> MPPGVDCPMEFWTKEENQSVVVDFLLPTGVYLNFPVSRNANLSTIKQLLWHRAQYEPLFHMLSGPEAYVFTCINQTAEQQELEDEQRRLCDVQPFLPVLRLVAREGDRVKKLINSQISLLIGKGLHEFDSLCDPEVNDFRAKMCQFCEEAAARRQQLGWEAWLQYSFPLQLEPSAQTWGPGTLRLPNRALLVNVKFEGSEESF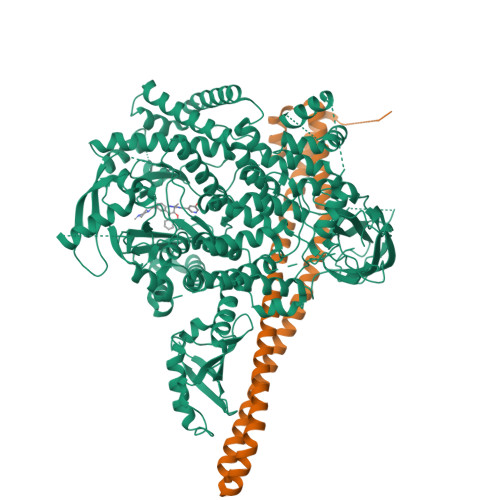TFQVSTKDVPLALMACALRKKATVFRQPLVEQPEDYTLQVNGRHEYLYGSYPLCQFQYICSCLHSGLTPHLTMVHSSSILAMRDEQSNPAPQVQKPRAKPPPIPAKKPSSVSLWSLEQPFRIELIQGSKVNADERMKLVVQAGLFHGNEMLCKTVSSSEVSVCSEPVWKQRLEFDINICDLPRMARLCFALYAVIEKAKKARSTKKKSKKADCPIAWANLMLFDYKDQLKTGERCLYMWPSVPDEKGELLNPTGTVRSNPNTDSAAALLICLPEVAPHPVYYPALEKILELGRHSECVHVTEEEQLQLREILERRGSGELYEHEKDLVWKLRHEVQEHFPEALARLLLVTKWNKHEDVAQMLYLLCSWPELPVLSALELLDFSFPDCHVGSFAIKSLRKLTDDELFQYLLQLVQVLKYESYLDCELTKFLLDRALANRKIGHFLFWHLRSEMHVPSVALRFGLILEAYCRGSTHHMKVLMKQGEALSKLKALNDFVKLSSQKTPKPQTKELMHLCMRQEAYLEALSHLQSPLDPSTLLAEVCVEQCTFMDSKMKPLWIMYSNEEAGSGGSVGIIFKNGDDLRQDMLTLQMIQLMDVLWKQEGLDLRMTPYGCLPTGDRTGLIEVVLRSDTIANIQLNKSNMAATAAFNKDALLNWLKSKNPGEALDRAIEEFTLSCAGYCVATYVLGIGDRHSDNIMIRESGQLFHIDFGHFLGNFKTKFGINRERVPFILTYDFVHVIQQGKTNNSEKFERFRGYCERAYTILRRHGLLFLHLFALMRAAGLPELSCSKDIQYLKDSLALGKTEEEALKHFRVKFNEALRESWKTKVNWLAHNVSKDNRQ;> YQQDQVVKEDNIEAVGKKLHEYNTQFQEKSREYDRLYEDYTRTSQEIQMKRTAIEAFNETIKIFEEQCQTQERYSKEYIEKFKREGNETEIQRIMHNYEKLKSRISEIVDSRRRLEEDLKKQAAEYREIDKRMNSIKPDLIQLRKTRDQYLMWLTQKGVRQKKLNEWLGN>GMLKLCGFAASNYYNKVKLALLEKNVPFEEVLAWIGETDTTATPAGKVPYMITESGSLCESEVINEYLEAAYPQTPLLPRDPMQAGKVREIVTFLELYLELTARELYPEAFFGGKVSDNVKERQLKLLSRYVPAFAKLAKFSPYVAGDTFTLADCAAAVHLPLVSSCTKIIYGKDLLADLPVKEYLKTLSERPSVQKVNADRKANTELMLSRN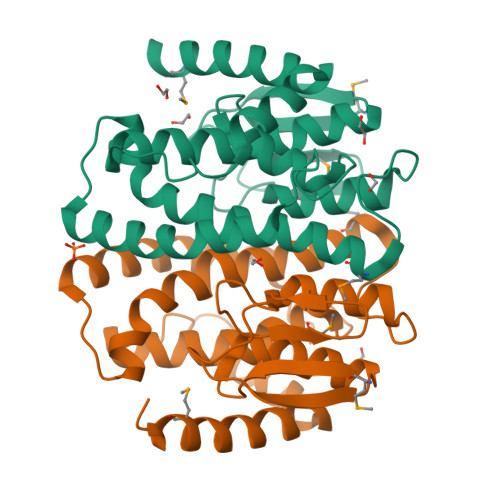K[2x]>MGSSHHHHHHSSGLVPRGSTSEVIEDEKQFYSKAKTYWKQIPPTVDGMLGGYGHISSIDINSSRKFLQRFLREGPNKTGTSCALDCGAGIGRITKRLLLPLFREVDMVDITEDFLVQAKTYLGEEGKRVRNYFCCGLQDFTPEPDSYDVIWIQWVIGHLTDQHLAEFLRRCKGSLRPNGIIV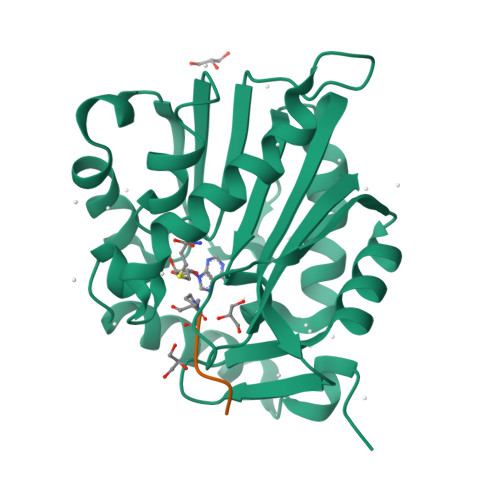IKDNMAQEGVILDDVDSSVCRDLDVVRRIICSAGLSLLAEERQENLPDEIYHVYSFALR[2x];>XPKRIA[2x]> GAMGMSTVHEILCKLSLEGDHSTPPSAYGSVKAYTNFDAERDALNIET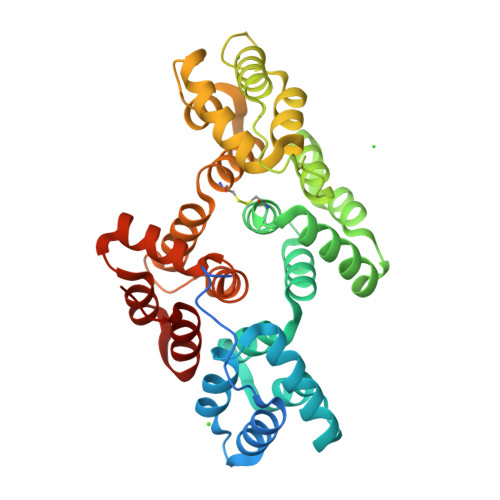AIKTKGVDEVTIVNILTNRSNEQRQDIAFAYQRRTKKELASALKSALSGHLETVILGLLKTPAQYDASELKASMKGLGTDEDSLIEIICSRTNQELQEINRVYKEMYKTDLEKDIVSDTSGDFRKLMVALAKGRRAEDGSVIDYELIDQDARDLYDAGVKRKGTDVPKWISIMTERSVCHLQKVFERYKSYSPYDMLESIKKEVKGDLENAFLNLVQCIQNKPLYFADRLYDSMKGKGTRDKVLIRIMVSRSEVDMLKIRSEFKKKYGKSLYYYIQQDTKGDYQKALLYLCGGDD> MSGSHHHHHHSGSMSPSPIEEQATRLLKEVPLIDGHNHFPYMIRGWFRNDINGQDAHLYDMPIGQTDLQRLQKGLLGGQFWSAFVPCPKNPDKEVGSLEALRQT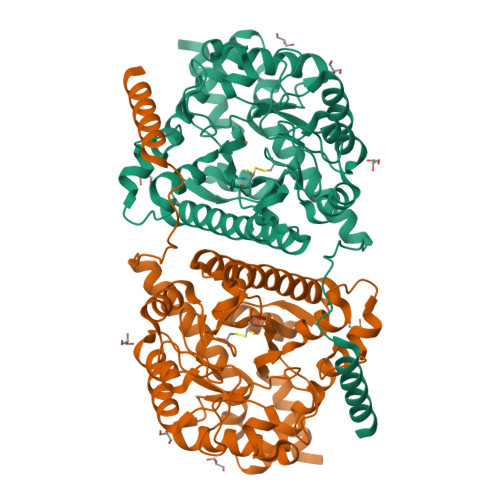LQQLDVIHRLIERHPTILQFADSAASIWSSFRAGRVASLIGIEGLHQIADSVSALRMLHRLGVRYVTLTHNCHNAFADAATVSPELHGGLSRKGERLIRELNRMGMMIDLSHTSHEAQTQALRLSRAPVIYSHSSIYSLRAHARNVTDENLHLLHRNRGVVMICFLRELLASEADQATLAHVIDHIIYAGTRIGYEHVGIGSDFDGMLRGPDGLHDVSCYPALVAGLLERGVSEEDVKRVMGLNVIRVLEEVERVAAELQGAGEECLCDELDEVWNEDIKEQLTRERERVRKLGPQK>[2x]MKVQYCDSLVIGGGLAGLRAAVATQQKGLSTIVLSLIPVKRSHSAAAQGGMQASLGNSKMSDGDNEDLHFMDTVKGSDWGCDQKVARMFVNTAPKAIRELAAWGVPWTRIHKGDRMAIINAQKTTITEEDFRHGLIHSRDFGGTKKWRTCYTADATGHTMLFAVANECLKLGVSIQDRKEAIALIHQDGKCYGAVVRDLVTGDIIAYVAKGTLIATGGYGRIYKNTTNAVVCEGTGTAIALETGIAQLGNME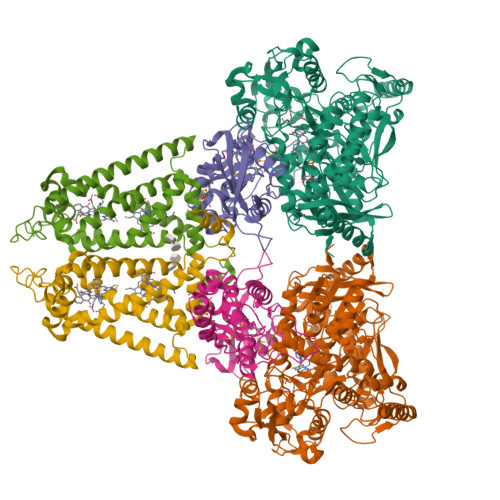AVQFHPTPLFPSGILLTEGCRGDGGILRDVDGHRFMPDYEPEKKELASRDVVSRRMIEHIRKGKGVQSPYGQHLWLDISILGRKHIETNLRDVQEICEYFAGIDPAEKWAPVLPMQHYSMGGIRTDYRGEAKLKGLFSAGEAACWDMHGFNRLGGNSVSEAVVAGMIVGEYFAEHCANTQVDLETKTLEKFVKGQEAYMKSLVESKGTEDVFKIKNRMKDVMDDNVGIFRDGPHLEKAVKELEELYKKSKNVGIKNKRLHANPELEEAYRVPMMLKVALCVAKGALDRTESRGAHNREDYPKRDDINWLNRTLASWPNPEQTLPTLEYEALDVNEMEIAPGYRGYGAKGNYIENPLSVKRQEEIDKIQSELEAAGKDRHAIQEALMPYELPAKYKARNERLGDK;>[2x]MGRMLTIRVFKYDPQSAVSKPHFQEYKIEEAPSMTIFIVLNMIRETYDPDLNFDFVCRAGICGSCGMMINGRPSLACRTLTKDFEDGVITLLPLPAFKLIKDLSVDTGNWFNGMSQRVESWIHAQKEHDISKLEERIEPEVAQEVFELDRCIECGCCIAACGTKIMREDFVGAAGLNRVVRFMIDPHDERTDEDYYELIGDDDGVFGCMTLLACHDVCPKNLPLQSKIAYLRRKMVSVN;>MTNESILESYSGVTPERKKSRMPAKLDWWQSATGLFLGLFMIGHMFFVSTILLGDNVMLWVTKKFELDFIFEGGKPIVVSFLAAFVFAVFIAHAFLAMRKFPINYRQYLTFKTHKDLMRHGDTTLWWIQAMTGFAMFFLGSVHLYIMMTQPQTIGPVSSSFRMVSEWMWPLYLVLLFAVILHGSVGLYRLAVKWGWFDGETPDKTRANLKKLKTLMSAFLIVLGLLTFGAYVKKGLEQTDPNIDYKYFDYKRTHHR[2x]>[2x]G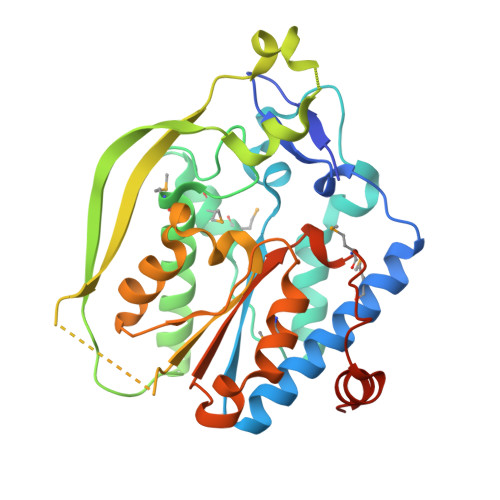SHMNEGRPGVVLGRDQWLFSDEEFKPTAGAEQLMQENLALIRGVRDTLQQHGSQLVLAIVPAKARVYTEYLGKERPASLHDDLYNQFHAQARQANVFAPDLMAPMEQAKARGQVFLRTDTHWTPMGAEVAAQALAEAVSRQSLLNGDPQAFITEAGNTAPYKGDLTNFLPLDPLFSNLLPAPDNLQKRTTRPVDAEGDAGDALFADKQIPVALVGTSYSANPHWNFLGALQQALRSDVANYAEDGHGPLLPMLKYLQSDAFKNAAPQVVVWEFPERYLPMKNDLSSFDPQWIAQLKNSRLEHHHHHH> SMIPDFMSFTSHIDELYESAKKQSGGKVADYIPQLAKFSPDLWGVSVCTVDGQRHSTGDTKV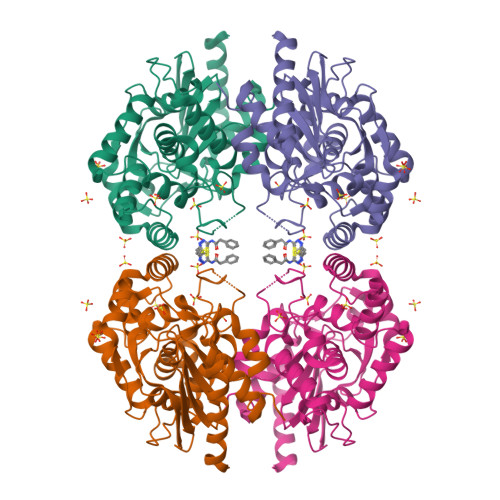PFCLQSCVKPLKYAIAVNDLGTEYVHRYVGKEPSGLRFNKLFLNEDDKPHNPMVNAGAIVVTSLIKQGVNNAEKFDYVMQFLNKMAGNEYVGFSNATFQSERESGDRNFAIGYYLKEKKCFPEGTDMVGILDFYFQLCSIEVTCESASVMAATLANGGFCPITGERVLSPEAVRNTLSLMHSCGMYDFSGQFAFHVGLPAKSGVAGGILLVVPNVMGMMCWSPPLDKMGNSVKGIHFCHDLVSLCNFHNYDNL> TRMCGSMSCPRNGCTCVYHWRRGHGCS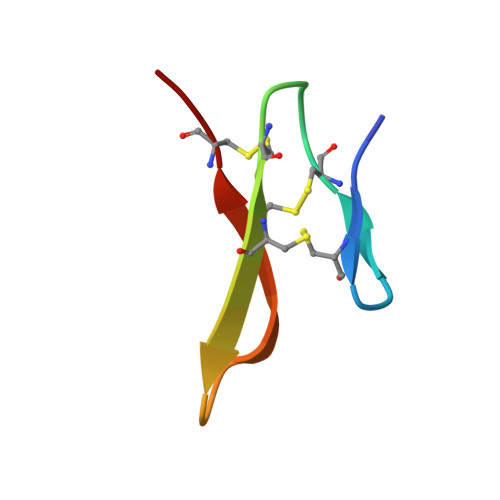CPG4-HYDROXY-3-METHOXYBENZOATE 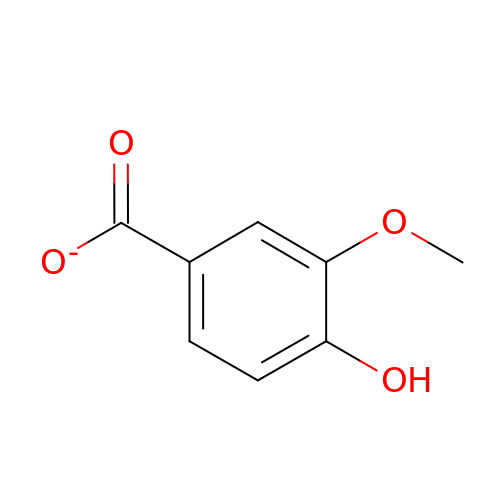| C8 H7 O4 | WKOLLVMJNQIZCI-UHFFFAOYSA-M>MSGMRFDTRLVHGGRRPSAGTGDVVPPIHVSTTYERRAQDEPRYFYGRGENPTREELEECLAGLERAPFATVFSSGQAAAATLLSLVRPGQCVVSTDDVYAGTDGLFDLAARQGVRVRYADLTTPEGIAAALAEPDLALVWIETPTNPLLTVVDVAEVSRRAHERGARVVVDNTFASPVLQQPLALGADVSLYSTTKSIAGHADVLGGALVYRDADLHAAVRAYRTTAGNVPGALDCFLVRRGLHTLSLRVHRQVATARVLVERLRASPVVGAVHYPGLPEHPQHAVVKAQMSAPGAIVSFDYLGGPAERLLDRFTLF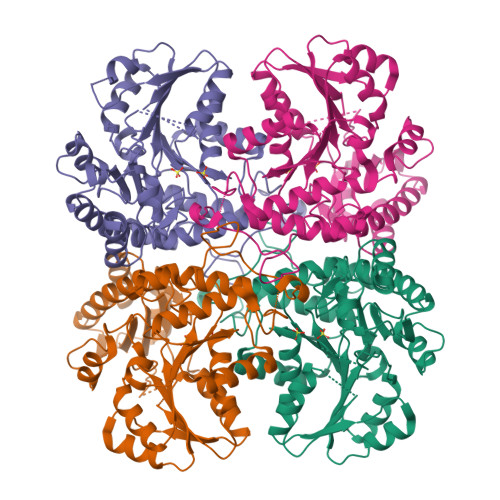TCGVSLGGVHSLVECPALMTHRPLSAEARARRGIGESLIRLSVGIEDPQDLAEDLSRALAGGTLEHHHHHH[8x]> RTIRYVRYESELQMPDIMRLITKDLSEPYSIYTYRYFIHNWPQL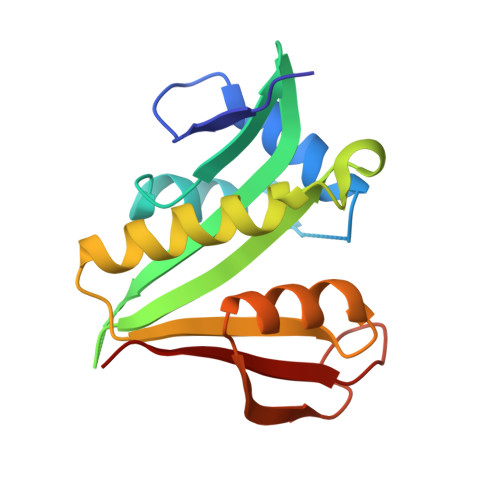CFLAMVGEECVGAIVCKLDMHKKMFRRGYIAMLAVDSKYRRNGIGTNLVKKAIYAMVEGDCDEVVLETEITNKSALKLYENLGFVRDKRLFRYYLNGVDALRLKLWLR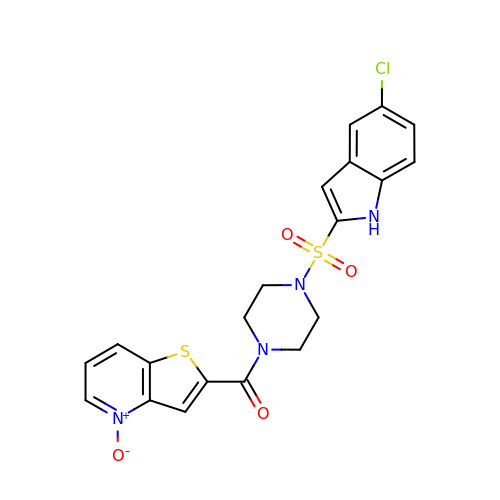2-({4-[(5-CHLORO-1H-INDOL-2-YL)SULFONYL]PIPERAZIN-1-YL}CARBONYL)THIENO[3,2-B]PYRIDINE 4-OXIDE | C20 H17 Cl N4 O4 S2 | DHDQMXPAANQKDC-UHFFFAOYSA-N> MSLNCERVWLNVTPATLRSDLADYGLLEPHALGVHEGRIHALVPMQDLKGPYPAHWQDMKGKLVTPGLIDCHTHLIFAGSRAEEFELRQK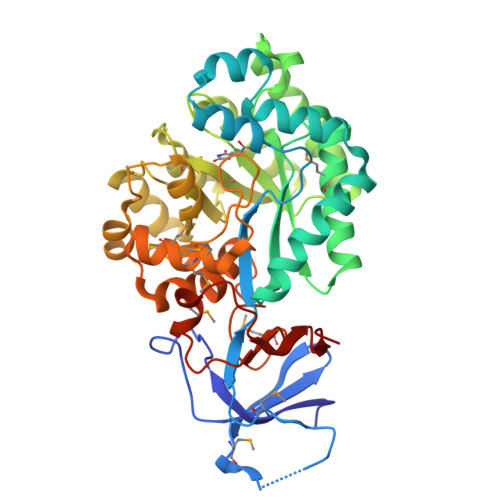GVPYAEIARKGGGIISTVRATRAASEDQLFELALPRVKSLIREGVTTVEIKSGYGLTLEDELKMLRVARRLGEALPIRVKTTLLAAHAVPPEYRDDPDSWVETICQEIIPAAAEAGLADAVDVFCEHIGFSLAQTEQVYLAADQYGLAVKGHMDQLSNLGGSTLAANFGALSVDHLEYLDPEGIQALAHRGVVATLLPTAFYFLKETKLPPVVALRKAGVPMAVSSDINPGTAPIVSLRMAMNMACTLFGLTPVEAMAGVTRHAARALGEQEQLGQLRVGMLADFLVWNCGHPAELSYLIGVDQLVSRVVNGEETLHGEGHHHHHH>VTAVVQRVEIHKLRQGENLILGFSIGGGIDQDPSQNPFSEDKTDKGIYVTRVSEGGPAEIAGLQIGDKIMQVNGWDMTMVTHDQARKRL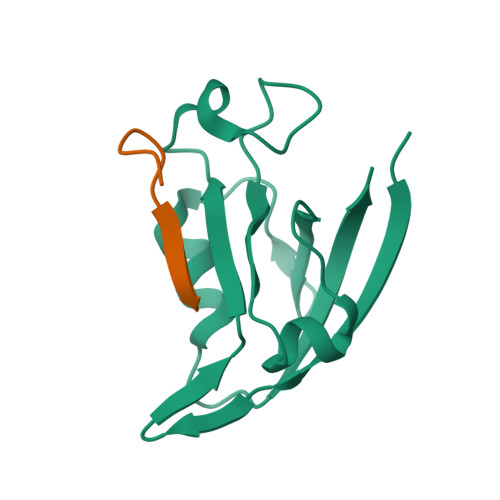TKRSEEVVRLLVTRQ[2x];>ANSRWPTSII[2x]> TLEGYYVDDALQGQGVYTYEDGGVLQGTYVDGELNGPAQEYDTDGRLIFKGQYKDNIRHGVCWIYYPDGGSLVGEVNEDGEMTGEKIAYVYPDERTALYGKFIDGEMIEGKLATLMSTEEGRPHFELMPG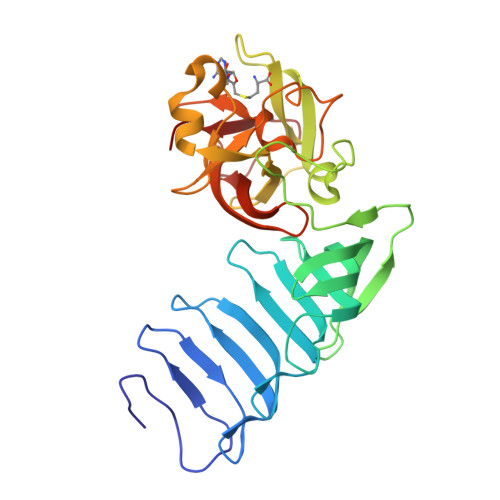NSVYHFDKSTSSCISTNALLPDPYESERVYVAESLISSAGEGLFSKVAVGPNTVMSFYNGVRITHQEVDSRDWALNGNTLSLDEETVIDVPEPYNHVSKYCASLGHKANHSFTPNCIYDMFVHPRFGPIKCIRTLRAVEADEELTVAYGY4-[4-(4-aminophenyl)buta-1,3-diyn-1-yl]-N-[(2S,3S)-3-hydroxy-1-nitroso-1-oxobutan-2-yl]benzamide 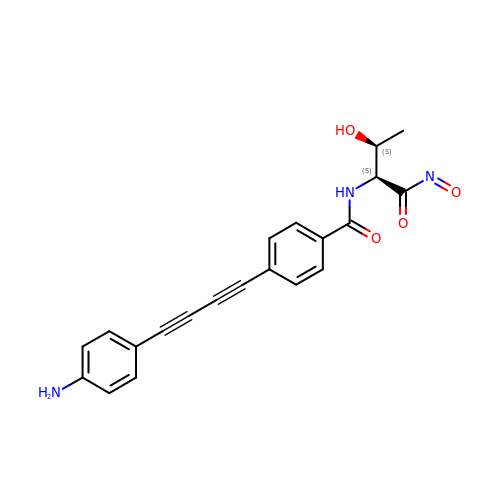| C21 H17 N3 O4 | DRMPSCRMGWDCMO-LIRRHRJNSA-N>GHMIDQLYRKAVLTVAERPQVEQLARQKMWNLAERFVAGESIESAIQAVQALERDGIAGNLDLLGEFIDSPAKCTEFADDVIKLIEAAHAAGIKPYVSIKLSSVGQGKDENGEDLGLTNARRIIAKAKEYGGFICLDMEDH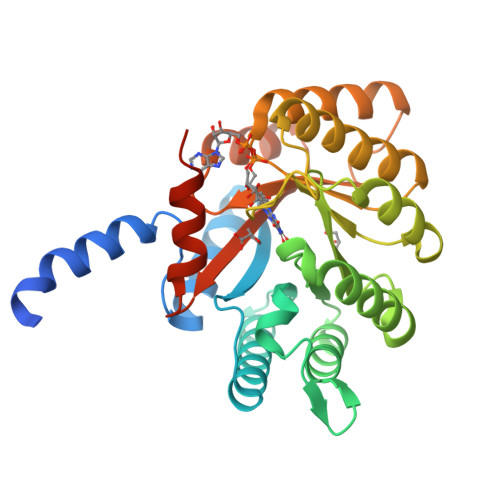TRVDVTLEQFRTLVGEFGAEHVGTVLQSYLYRSLGDRASLDDLRPNIRMVKGAYLEPATVAYPDKADVDQNYRRLVFQHLKAGNYTNVATHDERIIDDVKRFVLAHGIGKDAFEFQMLYGIRRDLQKQLAAEGYRVRVYLPYGRDWYAYFSRRIAETPRNAAFVVQGMLKG[2x]>MYKNVPIWAQKWKPTIKALQSINVKDLKIDPSFLNIIPDDDLTKSVQDWVYATIYSIAPELRSFIELEMKFGVIIDAKGPDRVNPPVSSQCVFTELDAHLTPNIDASLFKELSKYIRGISEVTENTGKFSIIESQTRDSVYRVGLSTQRPRFLRMSTDIKTGRVGQFIEKRHVAQLLLYSPKDSYDVKISLNLELPVPDNDPPEKYKSQSPISERTKDRVSYIHNDSCTRIDITKVENHNQNSKSRQSETTHEVELEINTPALLNAFDNITNDSKEYASLIRTFLNNGTIIRRKLSSLSYEIFEGSKKVM[2x];>[2x]SLMVLAMESRVAPEIPGLIQPGNVTQDLKMMVCKLLNSPKPTKTFPGSQPVSFQHSDVEE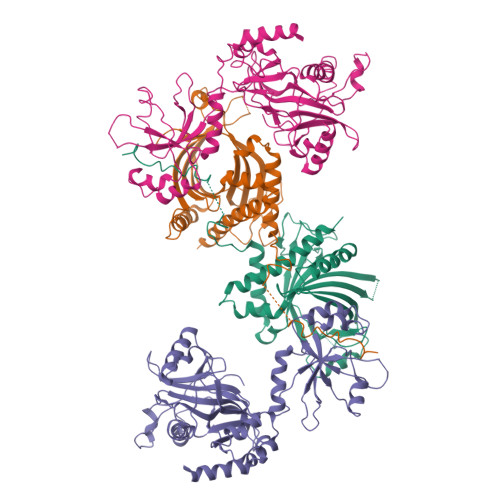KLLAHDYYVCEKTDGLRVLMFIVINPVTGEQGCFMIDRENNYYLVNGFRFPRLPQKKKEELLETLQDGTLLDGELVIQTNPMTKLQELRYLMFDCLAINGRCLTQSPTSSRLAHLGKEFFKPYFDLRAAYPNRCTTFPFKISMKHMDFSYQLVKVAKSLDKLPHLSDGLIFTPVKAPYTAGGKDSLLLKWKPEQENTVDFKLILDIPMVEDPSLPKDDRNRWYYNYDVKPVFSLYVWQGGADVNSRLKHFDQPFDRKEFEILERTYRKFAELSVSDEEWQNLKNLEQPLNGRIVECAKNQETGAWEMLRFRDDKLNGNHTSVVQKVLESINDSVSLEDLEEIVGDIKRCWDERRANMAGGSGRPLPSQSQNATLSTSKPVHSQPPSNDKEPKYVDEDDWSD>AIAMTHPDISVDVLVIGAGPTGLGAAKRLNQIDGPSWMIVDSNETPGGLASTDVTPEGFLYDVGGHVIFSHYKYFDDCLDEALPKEDDWYTHQRISYVRCQGQWVPAPFQNNISMLPKEEQVKCIDGMIDAALEARVANTKPKTFDEWIVRMMGTGIADLFMRPYNFKVWAVPTTKMQCAWLGERVAAPNLKAVTTNVILGKTAGNWGPNATFRFPARGGTGGIWIAVANTLPKEKTRFGEKGKVTKVNANNKTVTLQDGTTIGYKKLVSTMAVDFLAEAMNDQELVGLTKQLFYSSTHVIGVGVRGSRPERIGDKCWLYFPEDNCPFYRATIFSNYSPYNQPEASAALPTMQLADGSRPQSTEAKEGPYWSIMLEVSESSMKPVNQETILADCIQGLVNTEMLKPTDEIVSTYHRRFDHGYPTPTLEREGTLTQILPKLQDKD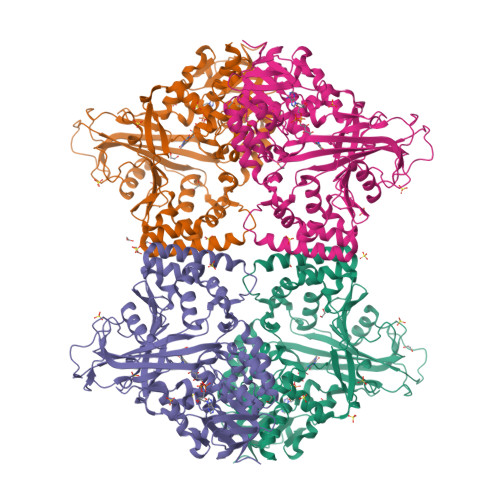IWSRGRFGSWRYEVGNQDHSFMLGVEAVDNIVNGAVELTLNYPDFVNGRQNTERRLVDGAQVFAKSKAQ[4x]> AGHMQQEAVAPEDSAVVKLATDSFNEYIQSHDLVLAEFFAPWCGHCKNMAPEYVKAAETLVEKNITLAQIDCTENQDLCMEHNIPGFPSLKIFKNSDVNNSIDYEGPRTAEAIVQFMIKQSQPAVAVVADLPAYLANETFVTPVIVQSGKIDADF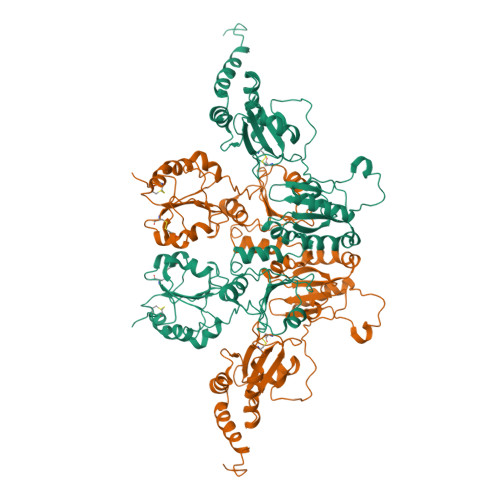NATFYSMANKHFNDYDFVSAENADDDFKLSIYLPSAMDEPVVYNGKKADIADADVFEKWLQVEALPYFGEIDGSVFAQYVESGLPLGYLFYNDEEELEEYKPLFTELAKKNRGLMNFVSIDARKFGRHAGNLNMKEQFPLFAIHDMTEDLKYGLPQLSEEAFDELSDKIVLESKAIESLVKDFLKGDASPIVKSQEIFENQDSSVFQLVGKNHDEIVNDPKKDVLVLYYAPWCGHCKRLAPTYQELADTYANATSDVLIAKLDHTENDVRGVVIEGYPTIVLYPGGKKSESVVYQGSRSLDSLFDFIKENGHFDVDGKALYEEAQEKAAEEADADAELADEEDAIHDEL>[2x]MAHHHHHHMSHYIELTEENFESTIKKGVALVDFWA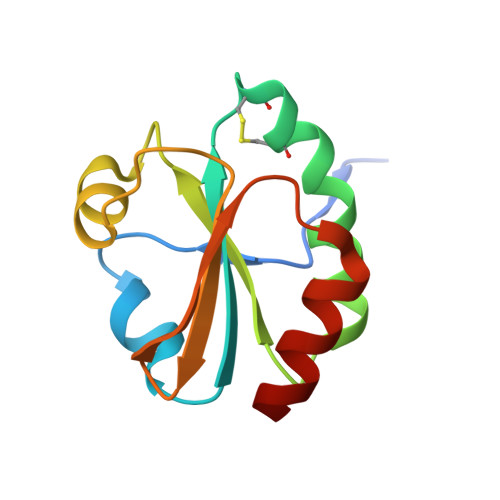PWCGPCKMLSPVIDELASEYQGKAKICKVNTDEQEELSAKFGIRSIPTLLFTKDGEVVHQLVGVQTKVALKEQLNKLLG> ALPQTVRIGTDTTYAPFSSKDAKGEFIGFDIDLGNEMCKRMQVKCTWVASDFDALIPSLKAKKIDAIISSLSITDKRQQEIAFSDKLYAADSRLIAAKGSPIQPTLESLKGKHVGVLQGSTQEAYANDNWRTKGVDVVAYANQDLIYSDLTAGRLDAALQDEVAASEGFLKQPAGKEYAFAGPSVKDKKYFGDGTGVGLRKDDTELKAAF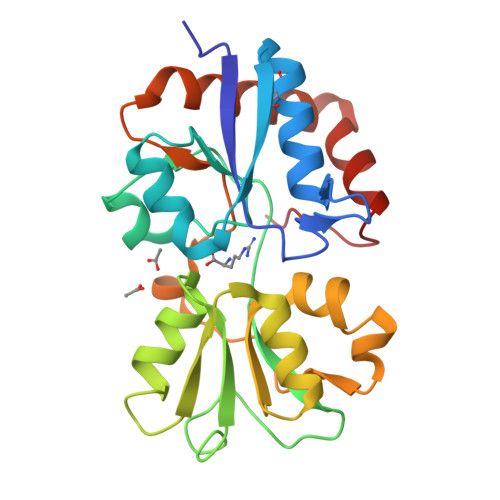DKALTELRQDGTYDKMAKKYFDFNVYGD>SNANTPQEAQQVDMWKKYIQWEKSNPLRTEDQTLITKRVMFAYEQCLLVLGHHPDIWYEAAQYLEQSSKLLAEKGDMNNAKLFSDEAANIYERAISTLLKKNMLLYFAYADYEESRMKYEKVHSIYNRLLAIEDIDPTLVYIQYMKFARRAEGIKSGRMIFKKAREDTRTRHHVYVTAALMEYYCSKDKSVAFKIFELGLKKYGDIPEYVLAYIDYLSHLNEDNNTRVLFERVLTSGSLPPEKSGEIWARFLAFESNIGDLASILKVEKRRFTAFKEEYEGKETALLVDRYKFMDLYPCSASELKALGYKDV[2x];>SNAMSAGEVERLVSELSGGTGGDEEEEWLYGDENEVER[2x]

In mammals, the cleavage and polyadenylation specificity factor (CPSF) constitutes the core of the 3′ end processing machinery onto which the remaining factors, including cleavage stimulation factor (CstF) and poly(A) polymerase (PAP), assemble. These interactions are mediated by Fip1, a CPSF subunit characterized by high degree of intrinsic disorder. Here, we report two crystal structures revealing the interactions of human Fip1 (hFip1) with CPSF30 and CstF77. Taken together, these results provide a structural basis for the multivalent scaffolding and regulatory functions of hFip1 in 3′ end processing.

To shed light on the hFip1–CstF77 interaction, we subsequently reconstituted a complex comprising the hFip11–35 fragment with a truncated construct of the CstF77 HAT domain (residues 241–549) and determined its X-ray crystallographic structure at a resolution of 2.7 Å. The structure reveals that hFip1 binds to a conserved positively charged patch located on the convex surface of the CstF77 HAT domain arch. Within the hFip11–35 fragment, only the evolutionarily conserved residues 20–27 were ordered, adopting an alpha-helical conformation. Interaction of hFip11–35 with CstF77 involves salt-bridge contacts of Glu22hFip1 and Glu23hFip1 with Arg402CstF77, and hydrophobic contacts involving Leu26hFip1 and Tyr27hFip1 with Phe398CstF77, Val428CstF77, Ile432CstF77, and Leu435CstF77. Additionally, the Tyr27hFip1 side chain interacts with Arg395CstF77 via π–π stacking. Corroborating these structural observations, simultaneous substitutions of Glu22hFip1 and Glu23hFip1, or Trp25hFip1, Leu26hFip1 and Tyr27hFip1 with alanine disrupted the hFip11–35–CstF7721–549 interaction in a pull-down experiment, whereas alanine substitution of Trp25hFip1 alone did not have an effect. In turn, mutation of the positively charged interaction surface in CstF77 (Arg395, Arg402, and Lys431 mutated to alanines) abolished the interaction with hFip11–35. Our crystal structure of the hFip1–CstF77 subcomplex reveals that a hFip1 binds via conserved motif within the N-terminal ‘acidic’ region to the convex arch of the CstF77 HAT domain on both protomers in the CstF77 homodimer, resulting in a 2:2 stoichiometry. By reanalysis of previously reported cryo-EM data, we reveal that this interaction mode is preserved in the context of the mPSF–CstF complex. In the presence of excess CstF77, PAP binding was considerably reduced, indicating that CstF77 competes with PAP for binding to hFip1.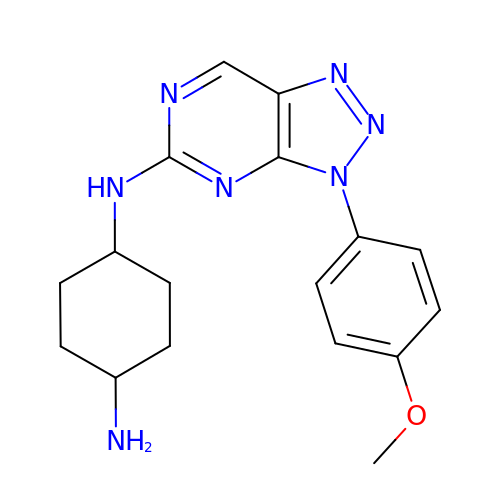~{N}4-[3-(4-methoxyphenyl)-[1,2,3]triazolo[4,5-d]pyrimidin-5-yl]cyclohexane-1,4-diamine | C17 H21 N7 O | OYCSZJFCBXZCDD-HAQNSBGRSA-N> GSMAKVQVNNVVVLDNPSPFYNPFQFEITFECIEDLSEDLEWKIIYVGSAESEEYDQVLDSVLVGPVPAGRHMFVFQADAPNPGLIPDADAVGVTVVLITCTYRGQEFIRVGYYVNNEYTETELRENPPVKPDFSKLQRNILASNPRVTRFHINWEDNT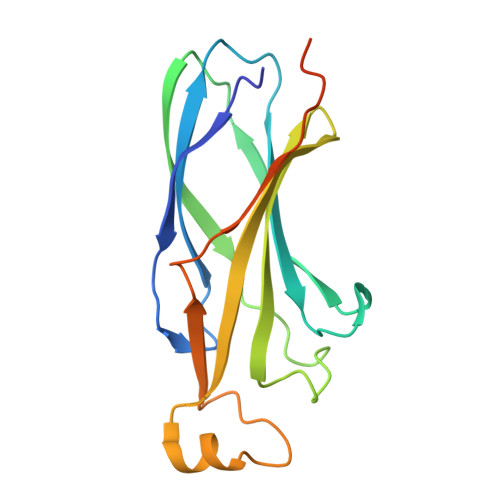EKLEDAESSNPNLQS>[2x]GSHMASMTGGQQMGRDPNMRILLAEDDLHLGEGLLEALQKEGLIVNLVSDGEAAQTFIESGLYDIVVLDIGMPIKTGLEVLRNIRNRGIKVPIILLTARDGL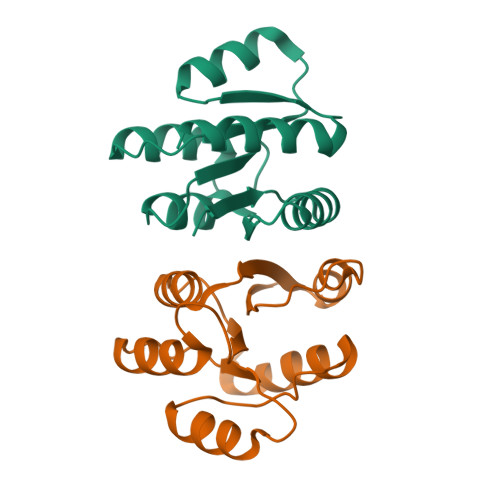EDRIKGLDLGADDYLTKPFELKELVARIKAISRRIDTRSGKS> SHHHHHHGESLFKGPRDYNPISSTICHLTNESDGHTTSLYGI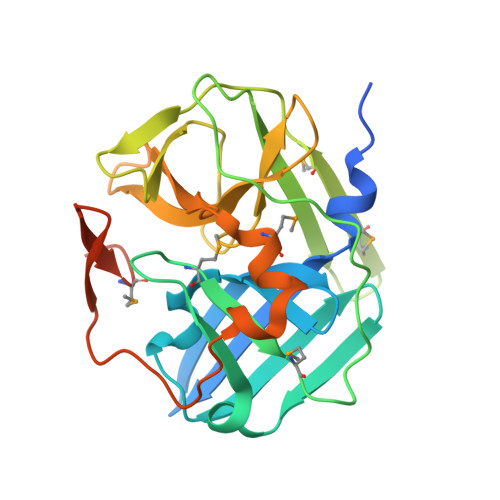GFGPFIITNKHLFRRNNGTLLVQSLHGVFKVKNTTTLQQHLIDGRDMIIIRMPKDFPPFPQKLKFREPQREERICLVTTNFQTKSMSSMVSDTSCTFPSSDGIFWKHWIQTKDGQAGSPLVSTRDGFIVGIHSASNFTNTNNYFTSVPKNFMELLTNQEAQQWVSGWRLNADSVLWGGHKVFMSKPEEPFQPVKEATQLMN ethyl 5-pyridin-4-yl-1~{H}-indole-2-carboxylate | C16 H14 N2 O2 | 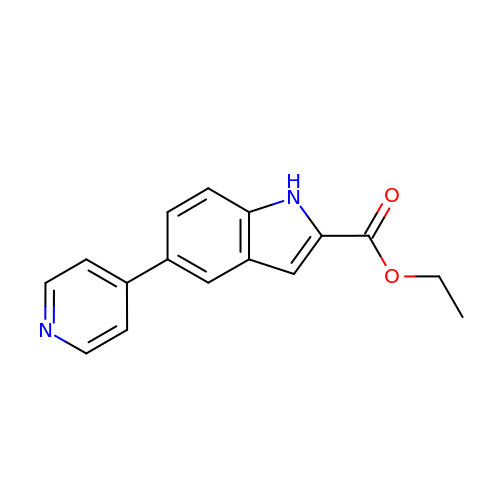HESNUJSXTQZPIZ-UHFFFAOYSA-N>[24x]SNAALN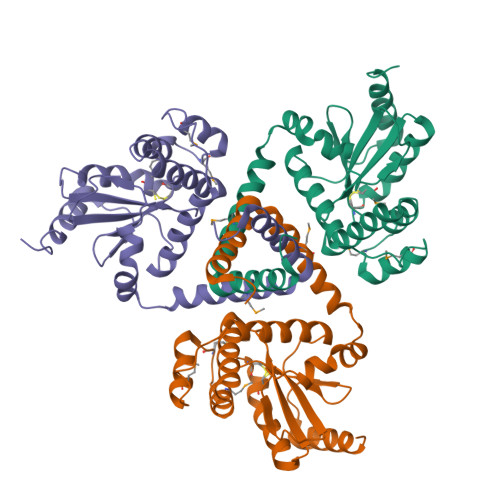AAQEKEVRALVRDTLVSNPEILEEAIMALQTKKADEQQAQFRQALASEHDALYNDAASPRIGAKDAKLVLVSFTDYNCPYCKRFDPLLEKITEQYPDVAVIIKPLPFKGESSAKASQAVLSVWKEDPKAFLALHQRLMQKKTMLDNASIEDAMKSTNTSKIKLTDDSLKTLQNNLELSRKLGIQGTPATVIGDTILPGAVDYDQLEIIVKEQLAKVKK4-(3'-amino[1,1'-biphenyl]-3-yl)-1H-pyrazol-5-amine | C15 H14 N4 | 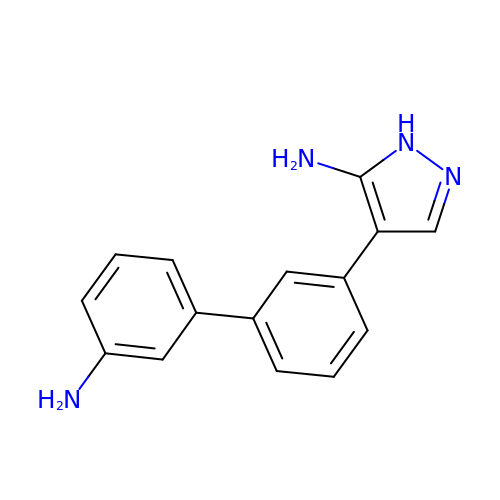XJQYSQDWCYFLKB-UHFFFAOYSA-N>MDIVDGDQCESNPCLNGGSCKDDINSYECWCPFGFEGKNCELLEHHHHHH[3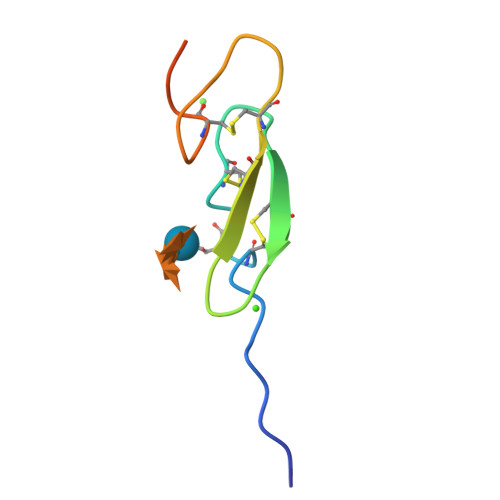x]>[2x]DSGCVVSWKNKELKCGSGIFITDNVHTWTEQYKFQPESPSKLASAIQKAHEEGICGIRSVTRLENLMWKQITPELNHILTENEVKLTIMTGDIKGIMQAGKRSLRPQPTELKYSWKAWGKAKMLSTELHNHTFLIDGPETAECPNTNRAWNSLEVEDYGFGVFTT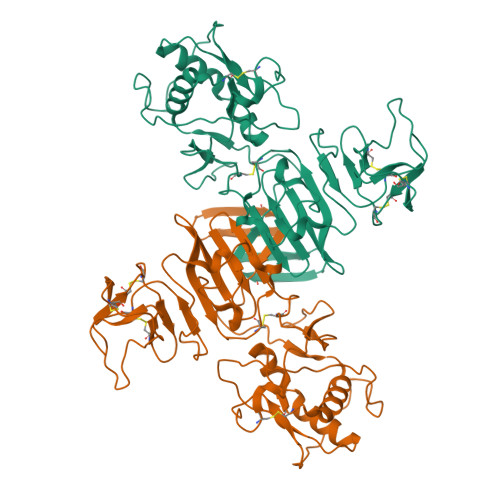NIWLKLKERQDVFCDSKLMSAAIKDNRAVHADMGYWIESALNDTWKIEKASFIEVKSCHWPKSHTLWSNGVLESEMIIPKNFAGPVSQHNYRPGYHTQTAGPWHLGRLEMDFDFCEGTTVVVTEDCGNRGPSLRTTTASGKLITEWCCRSCTLPPLRYRGEDGCWYGMEIRPLKEK N-[(4R)-1-(2-fluorophenyl)-4,5,6,7-tetrahydroindazol-4-yl]-2,1-benzoxazole-3-carboxamide 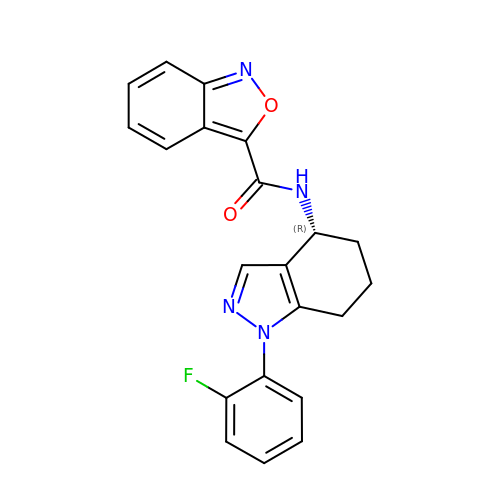| C21 H17 F N4 O2 | KVYFUACEMBMTLM-MRXNPFEDSA-N>ADPHKCDITLQEIIKTLNSLTEQKTLCTELTVTDI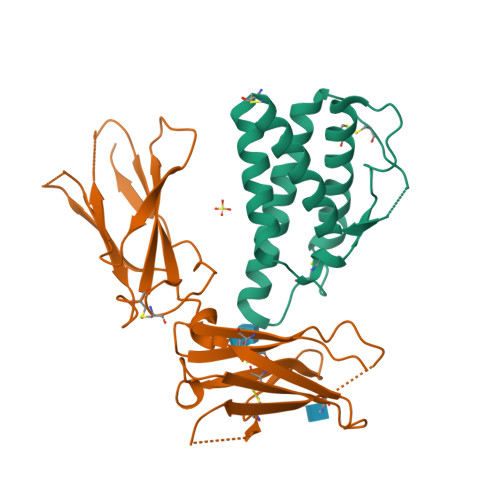FAASKNTTEKETFCRAATVLRQFYSHHEKDTRCLGATAQQFHRHKQLIRFLKRLDRNLWGLAGLNSCPVKEANQSTLENFLERLRVIMQSKWFKCGA[2x];>[2x]ADPLPLPEVQCFVFNVEYMNCTWQSSSEPQPTNLTLHYWYKNSDNDKVQKCSHYLFSEEITSGCQLQKKEIHLYQTFVVQLQDPREPRRQATQMLKLQNLVIPWAPENLTLHKLSESQLELNWNNRFLNHCLEHLVQYRTDWDHSWTEQSVDYRHKFSLPSVDGQKRYTFRVRSRFNPLCGSAQHWSEWSHPIHWGSNTSKEN> IGDEPLENYLDTEYFGTIGIGTPAQDFTVIFDTGSSNLWVPSVYCSSLACSDHNQFNPDDSSTFEATSQELSITYGTGSMTGILGYDTVQVGGISDTNQIFGLSETEPGSFLYYAPFDGILGLAYPSISASGATPVFDNLWDQGLVSQDLFSVYLSSNDDSGSVVLLGGIDSS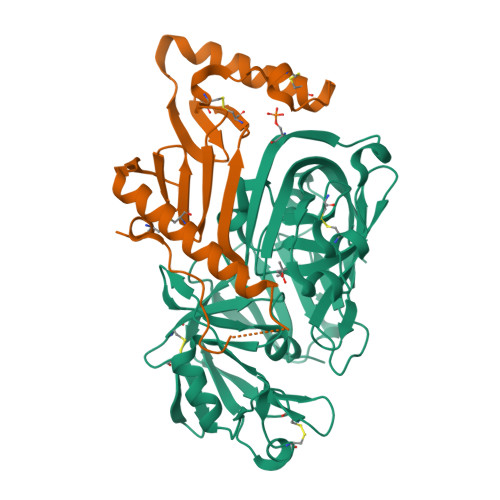YYTGSLNWVPVSVEGYWQITLDSITMDGETIACSGGCQAIVDTGTSLLTGPTSAIANIQSDIGASENSDGEMVISCSSIDSLPDIVFTINGVQYPLSPSAYILQDDDSCTSGFEGMDVPTSSGELWILGDVFIRQYYTVFDRANNKVGLAPVA;> QFLFSMSTGPFICTVKDNQVFVANLPWTMLEGDDIQVGKEFAARVEDCTNVKHDMAPTCTKPPPFCGPQDMKMFNFVGCSVLGNKLFIDQKYVRDLTAKDHAEVQTFREKIAAFEEQQENQPPSSGMPHGAVPAGGLSPPPPPSFCTVQ> MPMTVITLKNVPQSLRGDLTRWMQEIATGVYVGNFNSRIREYLWRRVQETMGAGEASMCFAARNELGYDFLTENASRSVIDYDGLP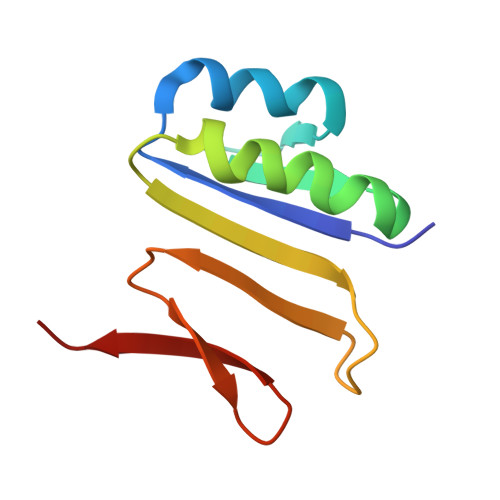LIFIPKE> 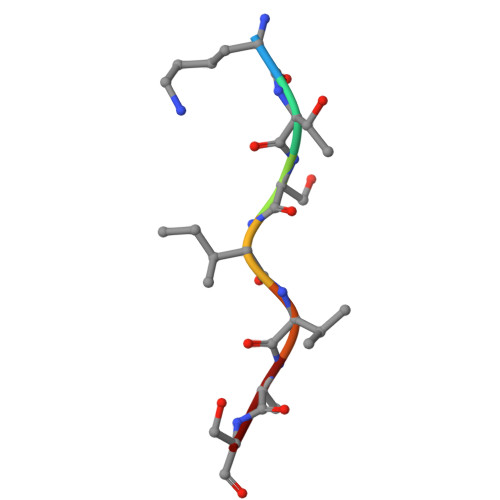KTSIVAS>M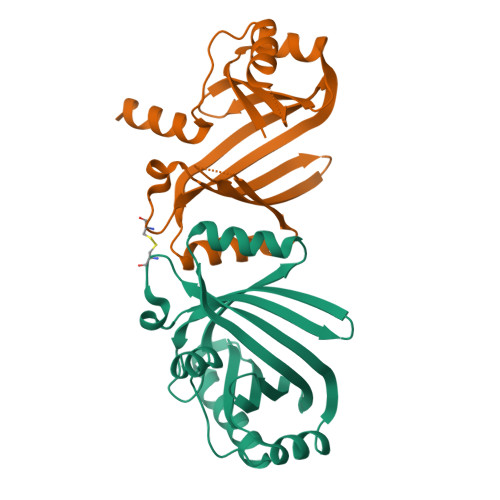YEVELKGYANDEIFEKVRETFEFMRKEIHEDIYYQHPCRDFSKTDEALRIRIKRFNGHNEVFLTYKGPKIDEKSKTRLEIEVEIQEDVDKYFELLDRLGFKEVLKVVKTREKYYVEKGVTITLDEVEGLGKFIEIETLVKEKDEIPEAVEKLEKILRELGVEKFERRSYLELLLEKRTELNI[2x]> GAACGACACTGACGAGGACTC;> TCGTCA;> TCGAGTCC;> GT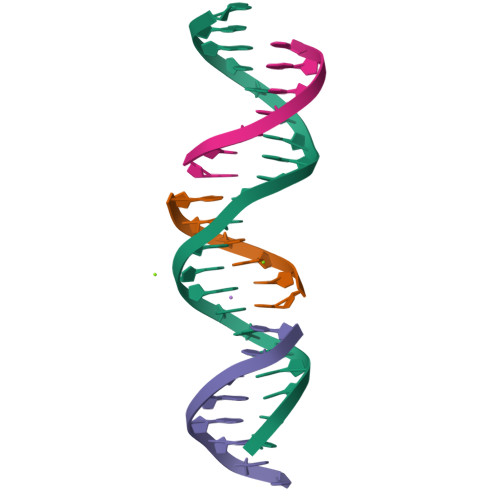GTCGT>[2x]MTPLGPASSLPQSFLLKCLEQVRKIQGDGAALQEKLCATYKLCHPEELVLLGHSLGIPWAPLSSCPSQALQLAGCLSQLHSGLFLYQGLLQALEGISPELGPTLDTLQLDVADFATTIWQQMEELGMAPALQPTQGAMPAFASAFQRRAGGVLVASHLQSFLEVSYRVLRHLAQP;>[2x]AGYPPASPSNLSCLMHLTTNSLVCQWEPGPETHLPTSFILKSFRSRADCQYQGDTIPDCVAKKRQNN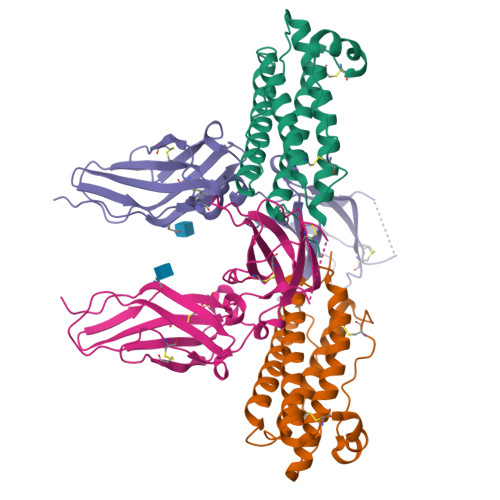CSIPRKNLLLYQYMAIWVQAENMLGSSESPKLCLDPMDVVKLEPPMLQALDIGPDVVSHQPGCLWLSWKPWKPSEYMEQECELRYQPQLKGANWTLVFHLPSSKDQFELCGLHQAPVYTLQMRCIRSSLPGFWSPWSPGLQLRPTMKA> GPLGSAYMSREESINPWILTGFADAEGSFLLRIRNNNKSSVGYSTELGFQITLHNKDKSILENIQSTWKVGVIANSGDNAVSLKVTRFEDLKVIIDHFEKYPLITQKLGDYMLFKQAFCVMENKEHLKINGIKELVRIKAKLNWGLTDELKKAFPEIISKERSLINKNIPNFKWLAGFTSGEGCFFVNLIKSKSKLGVQVQLVFSITQHIKDKNLMNSLITYLG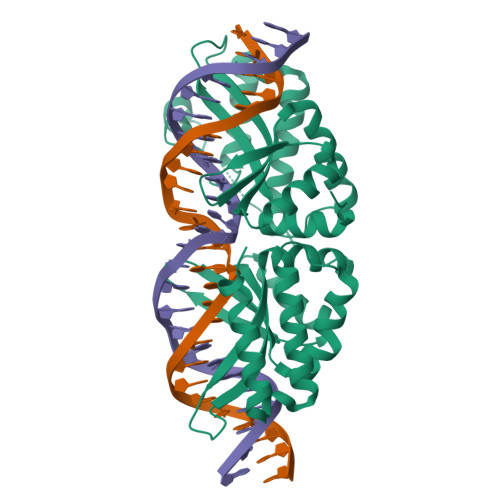CGYIKEYNKSEFSWLAFVVTKFSDINDKIIPVFQENTLIGVKLEDFEDWCKVAKLIEEKKHLTESGLDEIKKIKLNMNKGRVF> ATIKDVAKRANVSTTTVSHVINKTRFVAEETRNAVWAAIKELHYSPSAVARSLKVNHTKSIGLLATSSEAAYFAEIIEAVEKNCFQKGYTLILGNAWNNLEKQRAYLSMMAQKRVDGLLVMCSEYPEPLLAMLEEYRHIPMVVMDWGEAKADFTDAVIDNAFEGGYMAGRYLIERGHREIGVIPGPLERNTGAGRLAGFMKAMEEAMIKVPESWIVQGDFEPESGYRAMQQILSQPHRPTAVFCGGDIMAMGALCAADEMGLRVPQDVSLIGYDNVRNARYFTPALTTIHQPKDSLGETAFNMLLDRIVNKREEPQSIEVHPR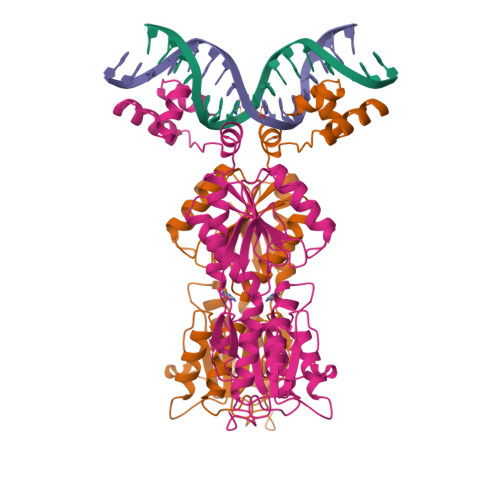LIERRSVADGPFRDYRR>MNKYTIAIDLGYGQIKGINQDNKRVIFPSIISSGKDRSLDTFFNSIDNIVDNIHVKILDEYFNEKEYFVGELAKRQPSNSSFINRDNKINSEENKVLLATALGLLIPNDLPNDTKIHIVTGLPLEHFIKQKQALNDMLKDFEHTIKFVDHNFSRNIKFEESNITLFPQGAGAIFSKINNDISSLLIKETFIGLIDVGFKTTDIVVFRINKDKEPVFEQEMSATLDGLGMINIYNTMDKAFTDNSRDGSKLNTEQLMLLCEEGKIFFKGDYIDLKKDLIKARK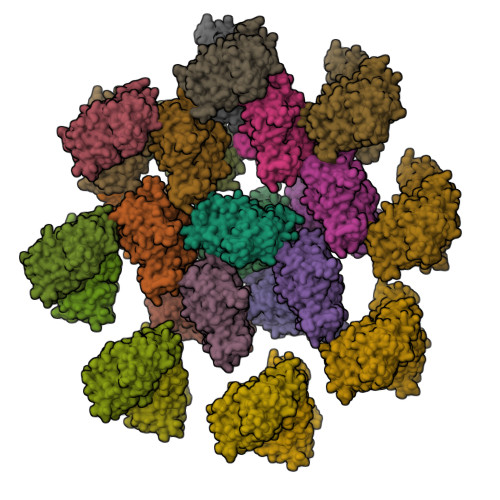TLSTNIINKADGLWGSRKNSFNSIMIAGGGGKVLYNHLKLIEPNMCQLIDNPEFANAIGYLEFGKQF[30x]> ARRPTICFRPINPSDLERLEQIHR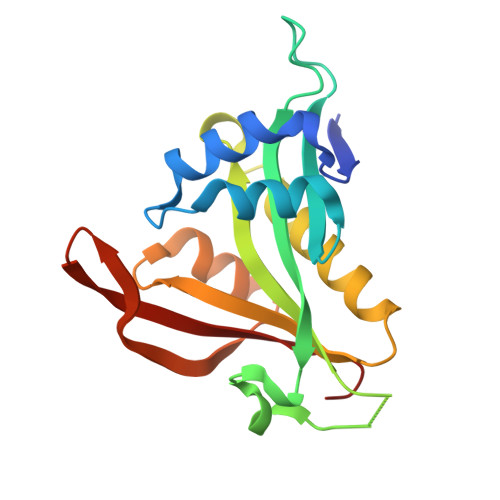DIFPIRYESEFFQNVVNGGDIVSWAAVDRSRPDGHSEELIGFVTAKIVLAKESEISDLIRYDSSKGEGTLVYILTLGVVETYRKRGIAKALINEVVKYSSGIPVCRGVYLHVIAHNNPAIRLYKRMSFRCVRRLHGFYLINGQHFDSYLFVYFINGS>[4x]RLTELREDIDAILEDPALEGAVSGVVVVDTATGEELYSRDGGEQLLPASNMKLFTAAAALEVLGADHSFGTEVAAESAPGRRGEVQDLYLVGRGDPTLSAEDLDAMAAEVAASGVRTVRGDLYADDTWFDSERLVDDWWPEDEPYAYSAQISALTVAHGERFDTGVTEVSVTPAAEGEPADVDLGAAEGYAELDNRAVTGAAGSANTLVIDRPVGTNTIAVTGSLPADAAPVTALRT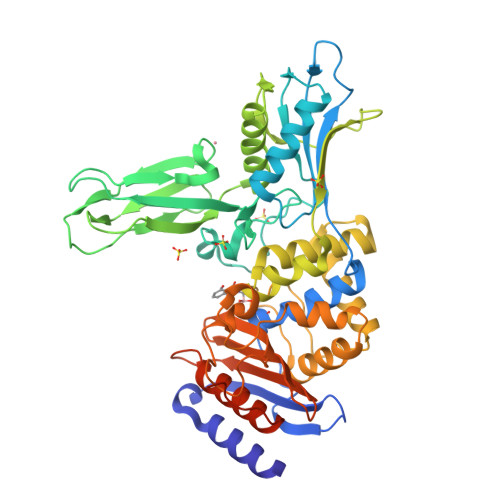VDEPAALAGHLFEEALESNGVTVKGDVGLGGVPADWQDAEVLADHTSAELSEILVPFMKFSNNGHAEMLVKSIGQETAGAGTWDAGLVGVEEALSGLGVDTAGLVLNDGSGLSRGNLVTADTVVDLLGQAGSAPWAQTWSASLPVAGESDPFVGGTLANRMRGTAAEGVVEAKTGTMSGVSALSGYVPGPEGELAFSIVNNGHSGPAPLAVQDAIAVRLAEYAGHQAPEGARMMRGPVQGSGELECSWVQAC The nuclear lamina is mainly composed of intermediate filament (IF) lamins and forms a protein-made meshwork that maintains the nuclear shape. Lamins consist of an alpha-helical central rod domain, an N-terminal head region, and a C-terminal long tail region. The basic building units of lamin filaments are coiled-coil dimers formed by parallel coiled-coil interactions between the central rod domains. The two basic building units are further assembled in an antiparallel manner by overlapping the coil 1b regions, called the “A11 tetramer”, as a polymerization intermediate.

The S143F mutation at LMNA exhibited mixed phenotypes of muscular dystrophy and progeroid syndrome with a deformed nuclear envelope structure, as observed in HGPS cells. The coiled-coil dimer of the S143F mutant lamin showed long alpha-helix bending at linker L1 between coil 1a and coil 1b. The mutated Phe143 is at the “c” position of the heptad repeat in coil 1b, orientating to the outside of the coiled-coil structure; thus, the mutation did not result in a substantial change in the coiled-coil structure of coil 1b. The crystallographic twofold symmetry built the A11 tetramer, showing the antiparallel arrangement of the two dimers by overlapping the coil 1b region. Furthermore, we confirmed that the S143F mutant lamin does not interfere with the A11 interaction in forming the linear filament since the A11 tetrameric structures between S143F and wild-type lamin A/C were similar overall, with an RMSD of 3.9 Å. Of note, the crystal structure of the S143F mutant lamin showed an X-shaped interaction between the two tetrameric units around Ala146 at the central residue of the tetramer. This X-shaped interaction between the A11 tetramers was not observed in the wild-type structure of the same lamin 300 fragment (Ahn, Jo et al. 2019). Of note, we found that the mutated Phe143 residues were clustered on the surface of the X-shaped structure with the surface-exposed leucine residues Leu140, Leu141, Leu148, and Leu152.

>TRLQEKEDLQELNDRLAVYIDRVRSLETENAGLRLRITESEEVVSREVSGIKAAYEAELGDARKTLDSVAKERARLQLELSKVREEFKELKARNTKKEGDLIAAQARLKDLEALLNFKEAALSTALSEKRTLEGELHDLRGQVAKLEAALGEAKKQLQDEMLRRVDAENRLQTMKEELDFQKNIYSEELRETKRRHETRLVEIA[2x]> RDFNNLTKGLCTINSWHIYGKDNAVRIGEDSDVLVTREPYVSCDPDECRFYALSQGTTIRGKHSNGTIHDRSQYRALISWPLSSPPTVYNSRVECIGWSSTSCHDGKTRMSICISGPNNNA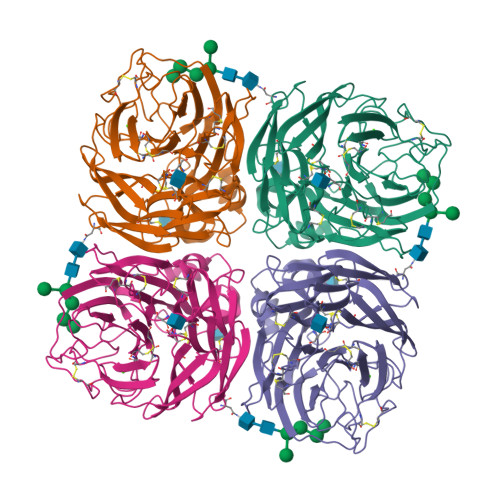SAVIWYNRRPVTEINTWARNILRTQESECVCHNGVCPVVFTDGSATGPAETRIYYFKEGKILKWEPLAGTAKHIEECSCYGERAEITCTCRDNWQGSNRPVIRIDPVAMTHTSQYICSPVLTDNPRPNDPTVGKCNDPYPGNNNNGVKGFSYLDGVNTWLGRTISIASRSGYEMLKVPNALTDDKSKPTQGQTIVLNTDWSGYSGSFMDYWAEGECYRACFYVELIRGRPNEDKVWWTSNSIVSMCSSTEFLGQWDWPDGAKIEYFL> MDMANQLLDELAHGNFSHLTLNLSQNGREIAILQKQLTGFDDKQLETFVEQHPAMPNDTRFKIMCTSFLNYARDVDPWSAWSSSDLIFE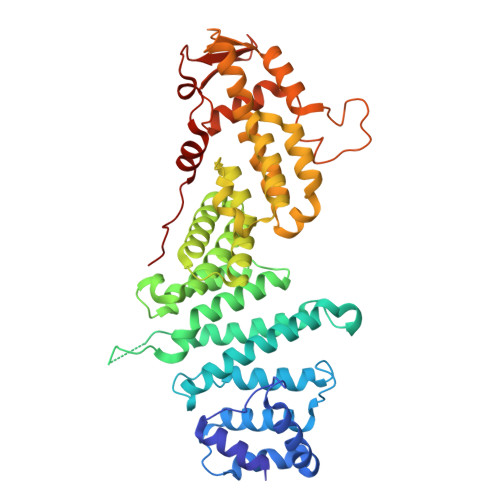FYQCLINCLINDNAPHIEMLIPVATRETEFIINLAGKLDSFHLQLHTRSHQFLSHISSILSRLFNSIKPPRGNASSTNIPGKQRILLYLVNKLNNIYFRIESPQLCSNIFKNFQPKSMLAHFNEYQLDQQIEYRYLLGRYYLLNSQVHNAFVQFNEAFQSLLNLPLTNQAITRNGTRILNYMIPTGLILGKMVKWGPLRPFLSQETIDNWSVLYKHVRYGNIQGVSLWLRQNERHLCARQLLIVLLEKLPMVTYRNLIKTVIKSWTTEWGQNKLPYSLIERVLQLSIGPTFEDPGAQEITIYNGIHSPKNVENVLVTLINLGLLRANCFPQLQLCVVKKTTMIQEIVPPVNERITKMFPAHSHVLW3-amino-5-(pyrrolidin-1-yl)-1H-pyrazole-4-carbonitrile | C8 H11 N5 | 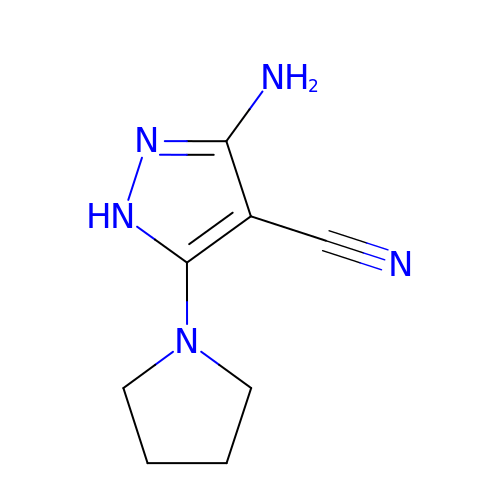RQDSNKYYHIZWJX-UHFFFAOYSA-N>[2x]MSLSNKIFTHSLPMRYADFPTLVDALDYAALSSAGMNFYDRRCQLEDQLEYQTLKARAEAGAKRLLSLNLKKGDRVALIAETSSEFVEAFFACQYAGLVAVPLAIPMGVGQRDSWSAKLQGLLASCQPAAIITGDEWLPLVNAATHDNPELHVLSHAWFKALPEADVALQRPVPNDIAYLQYTSGSTRFPRGVIITHREVMANLRAISHDGIKLRPGDRCVSWLPFYHDMG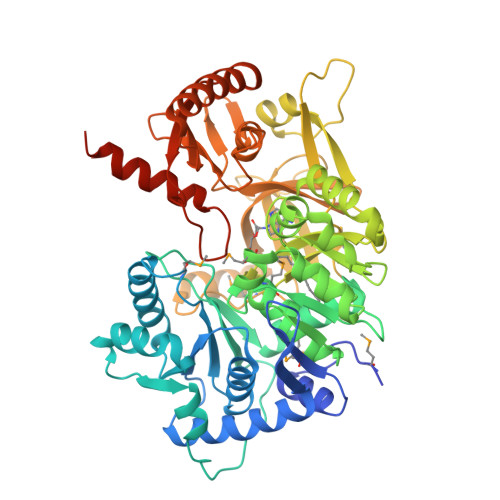LVGFLLTPVATQLSVDYLRTQDFAMRPLQWLKLISKNRGTVSVAPPFGYELCQRRVNEKDLAELDLSCWRVAGIGAEPISAEQLHQFAECFRQVNFDNKTFMPCYGLAENALAVSFSDEASGVVVNEVDRDILEYQGKAVAPGAETRAVSTFVNCGKALPEHGIEIRNEAGMPVAERVVGHICISGPSLMSGYFGDQVSQDEIAATGWLDTGDLGYLLDGYLYVTGRIKDLIIIRGRNIWPQDIEYIAEQEPEIHSGDAIAFVTAQEKIILQIQCRISDEERRGQLIHALAARIQSEFGVTAAIDLLPPHSIPRTSSGKPARAEAKKRYQKAYAASLNVQESLAEGHHHHHH>GGELMIKSSNAFDVIELSSQIQRYASLSKINNRTNPILKDNKAKEFKDADLKWLKLENCPTAGDVPTTGNNNDLQDQFIACDADYRKGDLSYFGSQFEFSTYVHPSNPEIQRQIKQVVSYFQYRGMERAFIGDAAGYVISEAKKKGFSAQDYRIVLIEPDRVGYFESNAISYEEFIENPSARENFLLKATKDRTLALAVSLAQTGEIAMQRDGSVAFLEDSELCWDTAAGSAKSCLSVRYDTVGNKTELDLKQIDVVSAKGLSFESDGKTKTPVVSTYETFQDGGRAKTINAIECPTGLNNRFAAVVSSFSTAGQNANFSSESAKDSQGTTQKDGSKGPHALLSGISLNWTLTNKVWDVTASIGIESGILPTSGIDSGSLLRNPKSLSFIAFQWCEN[6x];>[6x]FNDNYSSTSTVYATS

The toxin-coregulated pilus (TCP), an operon-encoded type IVb pilus (T4bP), plays a crucial role in this process, which requires an additional secreted protein, TcpF, encoded on the same TCP operon; however, its mechanisms of secretion and function remain elusive. Here, we demonstrated that TcpF interacts with the minor pilin, TcpB, of TCP and elucidated the crystal structures of TcpB alone and in complex with TcpF. Repetitive TcpA units form the filament structure, whereas TcpB displays multiple functions, such as efficient pilus assembly, pilus retraction, and CTXφ uptake. The structural analyses reveal how TCP recognizes TcpF and its secretory mechanism via TcpB-dependent pilus elongation and retraction.

We then analyzed the structure of TcpB alone and in complex with the TcpF (1–15) peptide. We used this TcpB structure as an MR search model to determine the TcpB and TcpF (1–15) peptide complex at a resolution of 2.30 Å. A structural model for all six peptides was successfully built, except for residues 12 to 15 on the C terminus due to the disorder of the region. TcpF (1–15) peptides can be recognized by clefts formed by TcpB domain 3, forming a unique hook-like conformation. A unique hook-like conformation, in which the five N-terminal residues of TcpF adopt a type I β turn structure stabilized by pi-pi stacking of the Phe1-Tyr5 pair, was recognized by the TcpB trimer. In forming this rather compact turn structure, the bulky aromatic amino acid pair got embedded in the binding pocket at the bottom of the clefts, with its N terminus firmly docked at β18 and β19 of TcpB via hydrogen bond interactions between the Phe1 amine group (TcpF) and the side chains of Ser373 and Ser388 (TcpB). The electrostatic interaction between Asp3 (TcpF) and Arg408 (TcpB), as well as the stacking interaction between Tyr5 (TcpF) and His366 (TcpB), further strengthened the rigidity of the turn structure. We speculate that the C terminus of TcpF (1–15) may help their NTDs efficiently come into contact to form a symmetrical trimer. With respect to TcpB and CofJ, although both their domain 3 structures adopt a similar H-type lectin-like fold, the length of the β13/β14 loop of TcpB, corresponding to the α4/β16 loop of CofB, is outstandingly short. This difference in the surface-exposed loop in TcpB makes it incapable of accommodating the elongated structure of CofJ T4bP-SS, which may explain the lack of binding between TcpB and CofJ.>SAASQAGSNYPRCWNCGGPWGPGREDRFFCPQCRALQAPDPTRDYFSLMDCNRSFRVDTAKLQHRYQQLQRLVHPDFFSQRSQTEKDFSEKHSTLVNDAYKTLLAPLSRGLYLLKLHGIEIPERTDYEMDRQF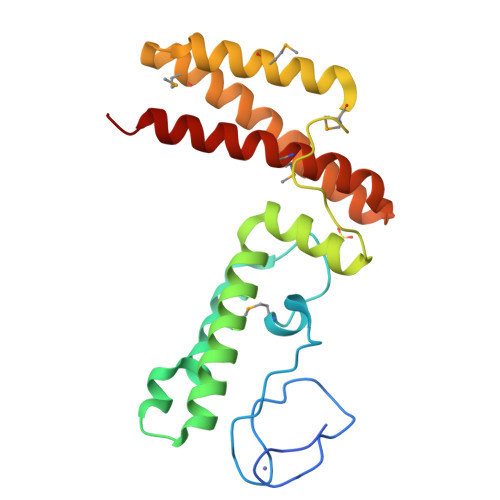LIEIMEINEKLAEAESEAAMKEIESIVKAKQKEFTDNVSSAFEQDDFEEAKEILTKMRYFSNIEEKIKLKKIPL[2x]>[2x]VSELSVATGAVSTASSSIPMPAGVNPADLAAELAAVVTESVDEDYLLYECDGQWVLAAGVQAMVELDSDELRVIRDGVTRRQQWSGRPGAALGEAVDRLLLETDQAFGWVAFEFGVHRYGLQQRLAPHTPLARVFSPRTRIMVSEKEIRLFDAGIRHREAIDRLLATGVREVPQSRSVDVSDDPSGFRRRVAVAVDEIAAGRYHKVILSRCVEVPFAIDFPLTYRLGRRHNTPVRSFLLQLGGIRA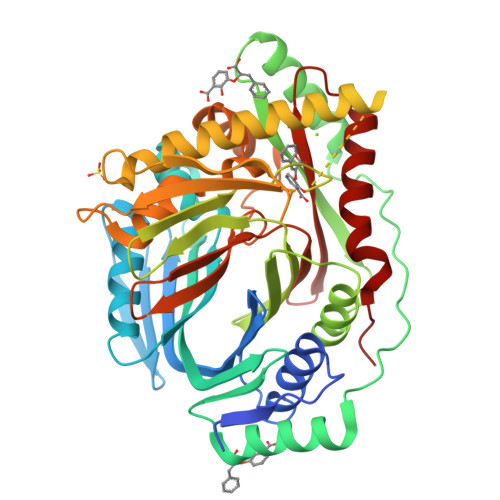LGYSPELVTAVRADGVVITEPLAGTRALGRGPAIDRLARDDLESNSKEIVEHAISVRSSLEEITDIAEPGSAAVIDFMTVRERGSVQHLGSTIRARLDPSSDRMAALEALFPAVTASGIPKAAGVEAIFRLDECPRGLYSGAVVMLSADGGLDAALTLRAAYQVGGRTWLRAGAGIIEESEPEREFEETCEKLSTLTPYLVARQ>GEGMWVPQQLPEIAGPLKKAGLKLSPQQISDLTGDPMGAVVALGGCTASFVSPNGLVVTNHACAYGAIQLNSTAENNLIKNGFNAPTTADEVSAGPNARVFVLDEITDVTKDAKAAIAAAGDDALARTKALEAFEKKLIADCEAEAGFRCRLYSFSGGNTYRLFKNLEIKDVRLAYAPPGSVGKFGGDIDNWMWPRHTGAFAFYRAYVGKDGKPAAFSKDNVPYQPKHWLKFADQPLGAGDFVMVAGYPGSTNRYALAAEFDNTAQWTYPTIARHYKNQIAMVEAAGKQNADIQVKYAATMAGWNNTSKNYDGQLEGFKRIDAAGQKLREEAAVLGWLKGQGAKGQPALDAHAKLLDLLEQSKATRDRDLTLALFNNTAMLGSATQLYRLSIEREKPNAERESGYQERDLPAIEGGLKQLERRYVAAMDRQLQEYWLNEYIKLPADQRVAAVDAWLGGNDAAAVKRALDRLAGTKLGSTEERLKW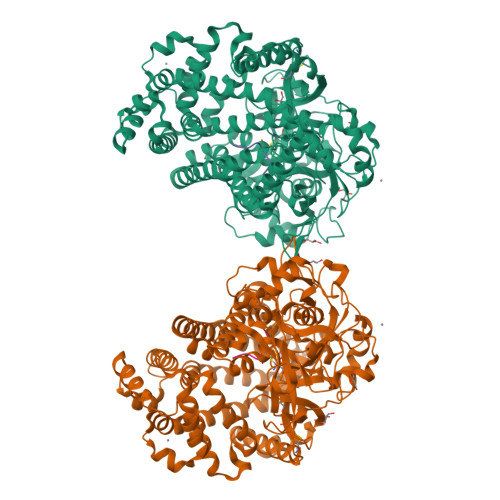FAADRKAFEASNDPAIQYAVAVMPTLLKLEQERKTRAGENLAARPVYLQALADYKKSQGEFVYPDANLSLRITFGNVMGYAPKDGMEYTPFTTLEGVVAKETGQDPFDSPKALLDAVAAKRYGGLEDKRIGSVPVNYLSDLDITGGNAGSPVLDAHGKLVGLAFDGNWESVSSNWVFDPKMTRMIAVDGRYLRWIMQEVYPAPQLLKEMNVGK[2x];>VYIHPF[2x]> ANIVGGIEYSINNASLCSVGFSVTRGATKGFVTAGHCGTVNATARIGGAVVGTFAARVFPGNDRAWVSLTSAQTLLPRVANGSSFVTVRGSTEAAVGAAVCRSGRTTGYQCGTITAKNVTANYAEGAVRGLTQGNACAGRGDSGGSWITSAGQAQGVMSGANVQSNGNNC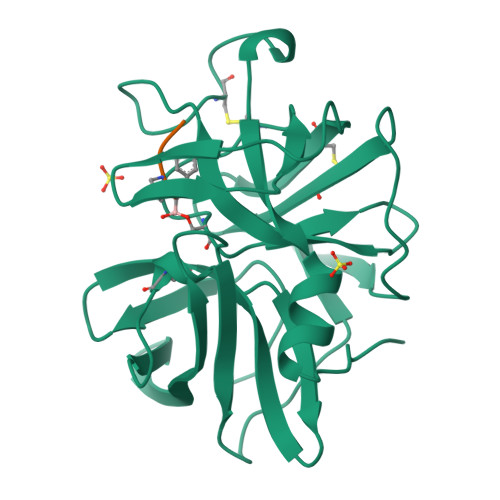GIPASQRSSLFERLQPILSQYGLSLVTG;> XAAPF> ARLGRQALLFPLCLVLYEFSTYIGNDMIQPGMLAVVEQYQAGIDWVPTSMTAYLAGGMFLQWLLGPLSDRIGRRPVMLAGVVWFIVTCLAILLAQNIEQFTLLRFLQGISLCFIGAVGYAAIQESFEEAVCIKITALMANVALIAPLLGPLVGAAWIHVLPWEGMFVLFAALAAISFFGLQRAMPETATRIGEKLSLKELGRDYKLVLKNGRFVAGALALGFVSLPLLAWTAQSPIIIITGEQLSSYEYGLLQVPIFGALIAGNLLLARLTSRRTVRSLIIMGGWPIMIGLLVAAAATVISSHAYLWMTAGLSIYAFGIGLANAGLVRLTLFASDMSKGTVSAAMEMLQMLIFTVGIEISKHAWLNGGNGLFNLFNLVNGILWLSLMVIFLK

A principal mechanism underpinning the unabated multidrug resistance is mediated by integral membrane proteins known as multidrug transporters. The majority of the known multidrug transporters utilize the inwardly directed H+ electrochemical gradient to expel drugs through cellular membranes. In sharp contrast to MdfA, which cannot extrude short dicationic compounds such as the neurotoxicant methyl viologen (MV), I239T/G354E can export both monocationic and short dicationic drugs, besides other well-known MdfA substrates. To answer these questions, we report the crystal structures of I239T/G354E in complexes with LDAO, MV and DXC, determined at resolutions up to 2.2 Å.

The best diffracting crystals of I239T/G354E were obtained in the presence of LDAO at pH 8. The resulting structure was determined to 2.2 Å resolution by combining molecular replacement and single wavelength anomalous dispersion (SAD) phasing. Overall, the LDAO-bound structure of I239T/G354E is similar to that of Q131R, which could be superimposed onto each other to yield a rms deviation of 1.0 Å for 390 common Cα atoms. This similarity suggested that our structure captures the transporter in an inward- or cytoplasm-facing state, and that the respective mutation gave rise to no global structural change even though I239T/G354E or Q131R reportedly altered the transport function. Perhaps unexpectedly, the density-modified SAD maps revealed two continuous, unbranched non-protein electron density features within I239T/G354E, indicating two bound LDAO molecules, denoted LDAO1 and LDAO2. LDAO1, similar to that seen in the LDAO-bound Q131R structure, is seated halfway into the lipid bilayer, at roughly equal distance between the extracellular and intracellular surfaces of the membrane. LDAO2, by contrast, is situated between LDAO1 and the cytoplasm-membrane interface, ~6 Å from the latter and appreciably more solvent-accessible than LDAO1. The closest approach of LDAO1 and LDAO2 exceeds 5 Å, implying that they interact with the transporter independently. Apparently, the addition of the side chain carboxylate of G354E, rather than substantial protein structural change, enables I239T/G354E to interact with a second LDAO molecule.> MLQLQRQKIIQDITQQIRS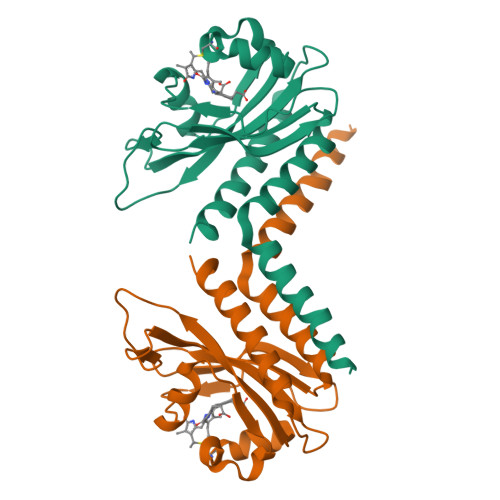TLNVNHILATVTQQVKELMQVERVIIFRLFPNGRSQIVEEVVSSEYAALKNYHWEDEKWSQEILDCYWQGKPRIVPDVINDIWTSCLVEYTTQGNIQSKIVAPILQELGENETGRWVSSEHKQKLWGVLVVHACSTKRVWEEDEAQLLQQIANQLAIAIQQLEHHHHHH> GPHMVKHPLNTAWTLWYTKPAVDKSESWSDLLRPVTSFQTVEEFWAIIQNIPEPHELPLKSDYHVFRNDVRPEWEDEANAKGGKWSFQLRGKGADIDELWLRTLLAVIGETIDEDDSQINGVVLSIRKGGNKFALWTASEDKEPLLRIGGK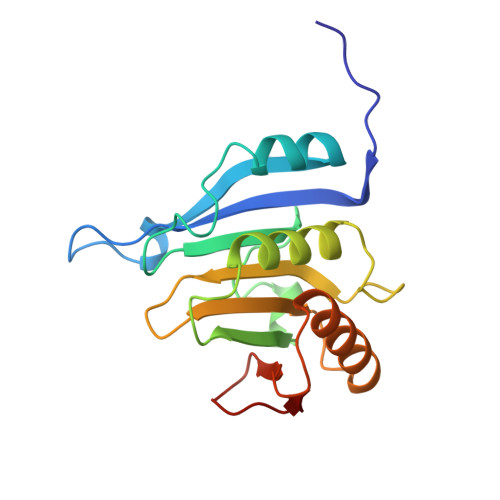FKQVLALTDDGHLEFFPHSSANGRHPQPSITL> MRMLSRNATFNSHGQDSSYFLGWQEYEKNPYHEVHNTNGIIQMGLAENQLCFDLLESWLAKNPEAAAFKKNGESIFAELALFQDYHGLPAFKKAMVDFMAEIRGNKVTFDPNHLVLTAGATSANETFIFCLADPGEAVLIPTPYYPGFDRDLKWRTGVEIVPIHCTSSNGFQITETALEEAYQEAEKRNLRVKGVLVTNPSNPLGTTMTRNELYLLLSFVEDKGIHLISDEIYSGTAFSSPSFISVMEVLKDRNCDENSEVWQRVHVV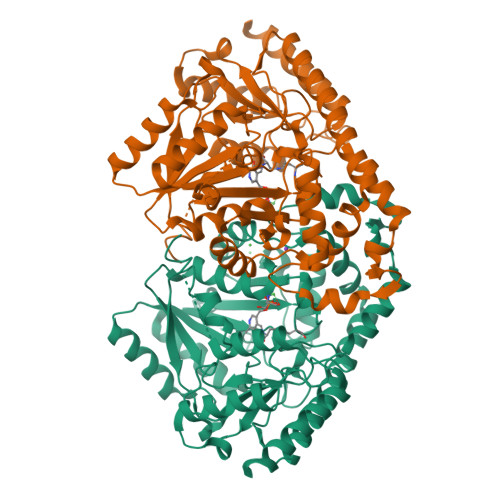YSLSKDLGLPGFRVGAIYSNDDMVVAAATKMSSFGLVSSQTQHLLSAMLSDKKLTKNYIAENHKRLKQRQKKLVSGLQKSGISCLNGNAGLFCWVDMRHLLRSNTFEAEMELWKKIVYEVHLNISPGSSCHCTEPGWFRVCFANLPERTLDLAMQRLKAFVGEYYNVPEVNGGSQSSHLSHSRRQSLTKWVSRLSFDDRGPIPGR Substituting His/Phe with Ser/Ile should expand the substrate-binding pocket to accommodate the bulkier substrate PET, and the strategy termed “double mutation (DM)” has proven to be useful to enhance PET hydrolytic activity of several IsPETase-like enzymes. Here, we report our experience in establishing the P. pastoris strain that expresses a PET hydrolytic enzyme from Caldimonas taiwanensis termed CtPL-DM that was identified from sequence mining from GenBank and modified by the DM strategy. In contrast to the protein expressed in Escherichia coli, CtPL-DM expressed in P. pastoris is inactive in PET degradation. Structural analysis indicates that a putative N-glycosylation site N181 could restrain the conformational change of a substrate-binding Trp and hamper the enzyme action.

We obtained the apo-form crystal structures of wild type and inactive variant S155A of CtPL-DM, which adopt the canonical α/β-hydrolase fold and are highly identical to the structure of IsPETase (Cα RMSD 0.477 Å and 0.471 Å). The TPA-binding W180 adopts the C-type conformation in the CtPL-DM structure and an alternative type in CtPL-DM-S155A. This suggests that DM strategy has conferred the TPA-binding Trp in CtPL-DM a wobble conformation. In both structures, a sugar that is covalently linked to N220 was observed. Protein sequence analysis indicates that there are three putative N-glycosylation sites in addition to N220 including N168, N181 and N261. N181 and N261 face towards the bulk solvent and could be glycosylated, despite no additional electron density map attached to these residues was observed. Notably, N181 is located adjacent to the TPA-binding residue W180, and its glycosylation, if any, could likely impose spatial hindrance to prevent W180 from wobbling and impact the substrate binding. Since the attempt to obtained substrate/analogue-bound complex failed, the MHET in IsPETase/MHET complex structure was modeled into these apo-form structures to investigate their substrate-binding modes. In all three structures, the TPA-binding W180 adopts conformations that should collide with the MHET. Nonetheless, W180 in F235L-S155A, which carries N181A mutation, shall be able to wobble freely. On the other hand, the conformational change of W180 in CtPL-DM and CtPL-DM-S155A is restrained by the glycosylated N181, thus impedes the binding of PET.

>[2x]EFNPYQKGPDPTASALERNGPFAIRSTSVSRTSVSGFGGGRLYYPTASGTYGAIAVSPGFTGTSSTMTFWGERLASHGFVVLVIDTITLYDQPDSRARQLKAALDYLATQNGRSSSPIYRKVDTSRRAVAGHAMGGGGSLLAARDNPSYKAAIPMAPWNTSSTAFRTVSVPTMIFGCQDDSIAPVFSSAIPIYNAIPNSTRKNYVEIRNDDHFCVMNGGGHDATLGKLGISWMKRFVDNDTRYSPFVCGAEYNRVVSSYEVSRSYNNCPY> ATTQIGEIVKTVANTVESEIKAELGVIPSLNAVETGATSNTEPEEAIQTRTVINMHGTAECLVENFLGRSALVCMRSFEYKNHSTSTSSIQKNFFIWTLNTRELVQIRRKMELFTYLRFDTEITIVPTLRLFSSSNVSFSGLPNLTLQAMYVPTGARKPSSQDSFEWQSACNPSVFFKINDPPARLTIPFMSINSAYANFYDGFAGFEKKATVLYGINPANTMGNLCLRVVNSYQPVQYTLTVRVYMKPKHIKAWAP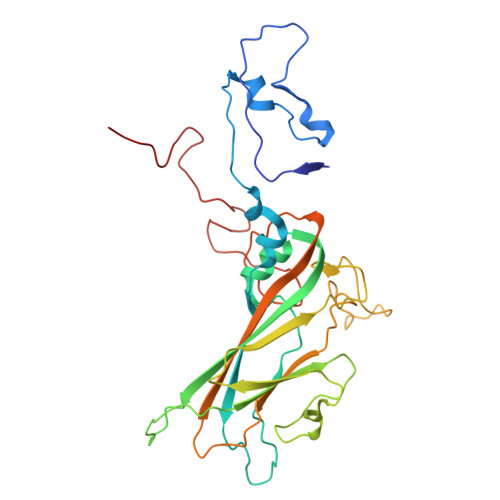RAPRTMPYTNILNNNYAGRSAAPNAPTAIVSHRSTIKTMPNDINLTTA As part of the RIKEN Structural Genomics Initiative (RSGI) project, in collaboration with UK Structural Genomics, we selected the hypothetical protein GK0453 (13 kDa, 113 residues) from Geo­bacillus kaustophilus HTA426 to predict its function from analysis of its crystal structure. The GK0453 protein is a member of the DUF1811 family in the Pfam database. In conclusion, the crystal structure of the hypothetical protein GK0453 revealed two small domains: a helix–turn–helix motif at the N-terminal region and an SH3-like β-barrel structure at the C-­terminal region. Based on structural comparisons, we speculate that the GK0453 protein may simultaneously interact with two proteins or with a protein and a nucleic acid to exert its unknown function.

The crystal structure of a conserved hypothetical protein, GK0453, from Geobacillus kaustophilus has been determined to 2.2 Å resolution. The crystal belonged to space group P43212, with unit-cell parameters a = b = 75.69, c = 64.18 Å. The N-terminal region contains a helix–turn–helix motif (α1, Lys14–Met34; α2, Val37–Tyr53). The C-terminal domain possesses a β-­barrel-like structure with four β-strands (β1, Glu64–Ile68; β2, Ala71–Lys82; β3, Phe85–Arg90; β4, Glu98–Pro101). All other results from the search showed that the structural similarity occurred within the distinct domains of either the 44-amino-acid N-­terminal region or the 54-amino-acid C-terminal region. Hence, we speculated from this analysis that the N-­terminal region of GK0453 may be involved in a protein–protein or a protein–nucleic acid interaction. Since the functional tetramerization and the critical residues for enzymatic function are absent in GK0453, it is unlikely that GK0453 possesses an activity similar to that of DHFR. The domain bearing these residues, which are responsible for recognizing the methylated histone tail, is absent in GK0453; however, the GK0453 and MRG15 chromodomain structures both possess similar hydrophobic environments. However, the structural analysis suggested that the β-barrel domain of GK0453 may also be involved in protein–protein interactions with an unknown function.

> GHMIKGEQKRYSEMTKEELQQEIAMLTEKARKAEQMGMVNEYAVYERKIAMAKAYMLNPADFHPGEIYEIEGAPGEYFKVRYLKGVFAWGWRLKGNGEEEALPISLLRKPNLPQS> MVPISPIETVPVKLKPGMDGPKVKQWPLTEEKIKALVEICTEMEKEGKISKIGPENPYNTPVFAIKKKDSTKWRKLVDFRELNKRTQDFWEVQLGIPHPAGLKKKKSVTVLDVGDAYFSVPLDEDFRKYTAFTIPSINNETPGIRYQYNVLPQGWKGSPAIFQSSMTKILEPFAAQ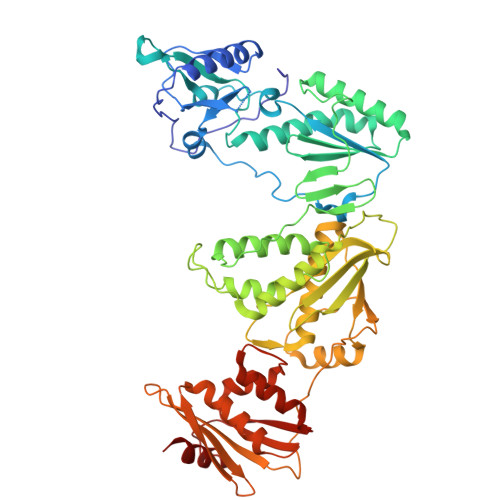NPDIVIYQYMDDLYVGSDLEIGQHRTKIEELRQHLLRWGLTTPDKKHQKEPPFLWMGYELHPDKWTVQPIVLPEKDSWTVNDIQKLVGKLNWASQIYPGIKVRQLSKLLRGTKALTEVIPLTEEAELELAENREILKEPVHGVYYDPSKDLIAEIQKQGQGQWTYQIYQEPFKNLKTGKYARMRGAHTNDVKQLTEAVQKITTESIVIWGKTPKFKLPIQKETWETWWTEYWQATWIPEWEFVNTPPLVKLWYQLEKEPIVGAETFYVDGAANRETKLGKAGYVTNKGRQKVVPLTNTTNQKTELQAIYLALQDSGLEVNIVTDSQYALGIIQAQPDKSESELVNQIIEQLIKKEKVYLAWVPAHKGIGGNEQVDKLVSA> ADTIVAVELDSYPNTDIGDPSYPHIGIDIKSVRSKSTARWNMQTGKVGTAHISYNSVAKR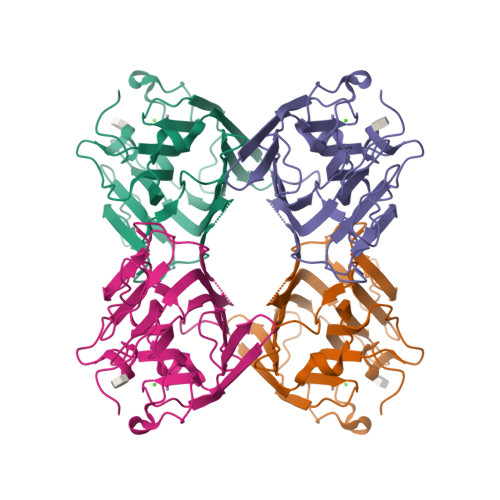LSAVVSYTGSSSTTVSYDVDLNNVLPEWVRVGLSATTGLYKETNTILSWSFTSKLKTNSIADANSLHFSFNQFSQNPKDLILQGDATTDSDGNLQLTRVSSDGSPQGSSVGRALFYAPVHIWEKSAVVASFDATFTFLIKSPDRDPADGITFFIANTDTSIPSGSGGRLLGLFPDAN>[2x]MGHHHHHHMMENKDALDIGKDDTNTSEADVSKNETQEQPVLSKSALKRLKRQQEWDAGREKRAEMRREKKRLRKEERKRKIEAGEVVKSQKKRIRLGKVVPSSIRIVLDCAFDDLMNDKEINSLCQQVTRCHSANRTALHPVELFATNFGGRLKTRQ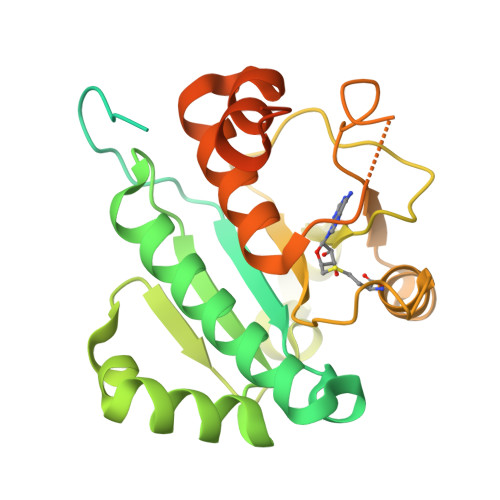DFVLKGQQNNWKRYNPTTKSYLEEFESQKEKLVYLSADSDNTITELDEDKIYIIGAIVDKNRYKNLCQNKASEQGIKTAKLPIDEYIKITDRKILTVNQVFEILSLWLEYRDWEKAFMEVIPKRKGILLKSDESFDVSEDTRSQSNQSDSELEKEN2-deoxy-beta-D-ribopyranose | C5 H10 O4 | 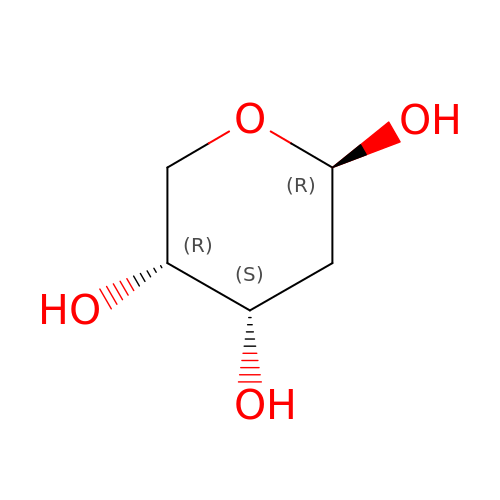ZVQAVWAHRUNNPG-VPENINKCSA-N> KKES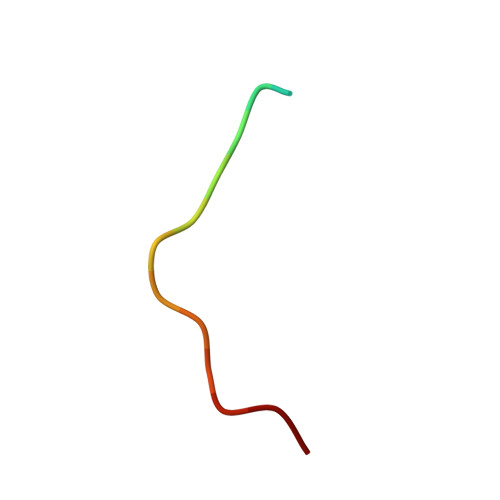RVVVWRLPPLH>MALVPVGMAPRQMRVNRCIFASIVSFDACITYKSPCSPDAYHDDGWFICNNHLIKRFKMSKMVLPIFDEDDNQFKMTIARHLVGNKERGIKRILIPSATNYQDVFNLNSMMQAEQLIFHLIYNNENAVNTICDNLKYTEGFTSNTQRVIHSVYATTKSILDTTNPNTFCSRVSRDELRFFDVTNARALRGGAGDQLFNNYSGFLQNLIRRAVAPEYLQIDTEELRFRNCATCIIDETGLVASVPDGPELYNPIRSSDIMRSQPNRLQIRNVLKFEGDTRELDRTLSGYEEYPTYVPLFLGYQIINSENNFLRNDFIPRANPNATLGGGAVAGPAPGVAGEAGGGIAV[12x];>MNDSNSLLITRLAAQILSRNMQTVDVIVDDKTLSLEEKIDTLTSMVLAVNSPPQSPPRVTSSDLAASIIKNNSKMVGNDFEMRYNVLRMAVVFVKHYPKYYNETTAGLVAEIESNLLQYQNYVNQGNYQNIEGYDSLLNKAEECYVKIDRLFKESIKKIMDDTEAFEREQEAERLRAEQTAANALLERRAQTSADDVVNRADANIPTAFSDPLPGPSAPRYMYESSESDTYMETARRTAEHYTDQDKDYNAAYTADEYNSLVKTVLLRLIEKALATLKNRLHITTIDQLKKFRDYLNSDADAGEFQIFLNQEDCVILKNLSNLASKFFNVRCVADTLEVMLEALRNNIELVQPESDAVRRIVIKMTQEIKDSSTPLYNIAMYKSDYDAIKNKNIKTLFDLYNDRLPINFLDTSATSPVRKTSGKRSAEDDLLPTRSSKRANRPEINVISSEDEQEDDDVEDVDYEKESKRRKLEDEDFLKLKALEFSKDIVNEKLQKIIVVTDGMKRLYEYCNCKNSLETLPSAANYGSLLKRLNLYNLDHIEMNVNFYELLFPLTLYNDNDNSDKTLSHQLVNYIFLASNYFQNCAKNFNYMRETFNVFGPFKQIDFMVMFVIKFNFLCDMRNFAKLIDELVPNKQPNMRIHSVLVMRDKIVKLAFSNLQFQTFSKKDKSRNTKHLQRLIMLMNANYNVI[6x];>MKRIKCNKVRTVTEIVNSDEKIQKTYELAEFDLKNLSSLESYETLKIKLALSKYMAMLSTLEMTQPLLEIFRNKADTRQIAAVVFSTLAFIHNRFHPLVTNFTNKMEFVVTETNDTSIPGEPILFTENEGVLLCSVDRPSIVKMLSREFDTEALVNFENDNCNVRIAKTFGASKRKNTTRSDDYESNKQPNYDMDLSDFSITEVEATQYLTLLLTVEHAYLHYYIFKNYGVFEYCKSLTDHSLFTNKLRSTMSTKTSNLLLSKFKFTIEDFDKINSNSVTSGFNIYNFNK[6x];>MSAIALYLEINKLRLKIDEPMQLAIWPQLFPLLCDEHQSVQLNTDVLINFMMHVARKSQNTILNNNAAIASQYAAGNADVVAAPASAQPTPRPVINLFARANAAAPAQPSEELINMRRYRNAARKLIHHYSLNSTSSTEYKISDVVMTMIFLLRSEKYHSLFKLLETTFDDYTCRPQMTQVQTDTLLDAVRSLLEMPSTTIDLTTVDIMRSSFARCFNSPIMRYAKIVLLQNVALQRDKRTTLEELLIERGEKIQMLQPQQYINSGTEIPFCDDAEFLNRLLKHIDPYPLSRMYYNAANTMFYTTMENYAVSNCKFNIEDYNNIFKVMENIRKHSNKNSNDQDELNIYLGVQSSNAKRKKY[6x];>MECPFQIQVCISDRFFAFPHNLVEPQSDVGNKLIENLIVYVPTDDDRLYIDKKQFPKFNSVLVYRHEHDVNIDSRSPKKTASATIVYWNPLVPITEIGAGETRVFSVLLTNNLFYCNTMIVHHENPKCPIEFTYPETDMQSACSALLKNRNGQSVPPPIKSNLRPIACEIPLSHFKELVESNDFLLCFNLETSTMVKILSLKRIFCIFQYRKQPARYVINLPHEEIDNLYNKLNWERTRRLMKGDVPSNCATVNRSSLKYIKQAQSLLGIPDYSQTVVDFVKMFQKIIFPYQLVPNVIIKLNNFDQMVSSAPNKAEPYKKIRLFCKNDSIAISSSGIVPINMPDFSPPNTFDYSDYANRTNINFVTQRVLTDGGFSSGITVTPVKYNYYL[2x];>[2x]MSGGGNLLTLERDHFKYLFLTSYFDLKDNEHVPSEPMAFIRNYLNCTFDLLDDAVLMNYFNYLQSMQLKHLVGSTSTNIFKFVKPQFRFVCDRTTVDILEFDTRMYIKPGTPVYATNLFTSNPRKMMAFLYAEFGKVFKNKIFVNINNYGCVLAGSAGFLFDDAYVDWNGVRMCAAPRLDNNMHPFRLYLLGEDMAKHFVDNNILPPHPSNAKTRKINNSMFMLKNFYKGLPLFKSKYTVVNSTKIVTRKPNDIFNEIDKELNGNCPFIKFIQRDYIFDAQFPPDLLDLLNEYMTKSSIMKIITKFVIEENPAMSGEMSREIILDRYSVDNYRKLYIKMEITNQFPVMYDHESSYIFVSKDFLQLKGTMNAFYAPKQRILSILAVNRLFGATETIDFHPNLLVYRQSSPPVRLTGDVYVVDKNEKVFLVKHVFSNTVPAYLLIRGDYESSSDLKSLRDLNPWVQNTLLKLLIPDSVQ;>[2x]MASSLQSKWICLRLNDAIIKRHVLVLSEYADLKYLGFEKYKFFEYVIFQFCNDPQLCKIIENNYNYCMQIFKAPADDMRDIRHNIKRAFKTPVLGHMCVLSNKPPMYSFLKEWFLLPHYKVVSLKSESLTWGFPHVVVFDLDSTLITEEEQVEIRDPFVYDSLQELHEMGCVLVLWSYGSRDHVAHSMRDVDLEGYFDIIISEGSTVQEERSDLVQNSHNAIVDYNLKKRFIENKFVFDIHNHRSDNNIPKSPKIVIKYLSDKNVNFFKSITLVDDLPTNNYAYDFYVKVKRCPTPVQDWEHYHNEIIQNIMDYEQYFIK

To understand the provenance and biology of baculo-like viruses, we have determined the structure of the nucleocapsid in the intact BV of the prototypical baculovirus, Autographa californica multiple nucleopolyhedrovirus (AcMNPV). Using cryo–electron microscopy, we show that the nucleocapsid forms a covalently cross-linked helical tube protecting a highly compacted 134-kilobase pair DNA genome. The ends of the tube are sealed by the base and cap substructures, which share a 126-subunit hub but differ in components that promote actin tail–mediated propulsion and nuclear entry of the nucleocapsid, respectively. The nucleocapsid orchestrates key steps in the infection cycle including the packaging of the genome, membrane envelopment, actin tail–driven trafficking within the cells, and breach of the nuclear pore upon genome delivery.

The hub forms a ring with a 14-fold rotational symmetry (C14) consisting of five proteins that have various names in the literature for historical reasons. Here, we rename them Hub1 (ODV/BV-C42 or AC101), Hub2 (ODV-EC27 or AC144), Hub3 (VP80 or AC104), HSP1 (hub spike protein 1, AC109), and HSP2 (hub spike protein 2, AC142) according to their functions. Hub1 and Hub2 form an intricate complex, with the compact Hub2 at its core and a series of helices in the C terminus of Hub1 (D3239-350) wrapping around most of Hub2. In the base, but not the cap, the hub accommodates a large chamber-like structure that forms a “plug” (bottom middle). Like the core of the hub, the plug is composed of Hub1-Hub2 complexes. Relative to the Hub2 orientation in the hub, the inner Hub2 subunit rotates by 162° toward the central axis of the particle due to a sharp kink in the handle of the other Hub2 subunit. This conformational shift effectively closes the chamber-like structure, sealing the basal end of the nucleocapsid. The inner side of the hub is decorated by 14 copies of the baculovirus C-terminal domain (CTD) phosphatase (BCP; also known as 38K or AC98) protein, which was not known to be a structural component of the nucleocapsid before an independent structure of the ODV. Sequence and structural analyses identify BCP as a member of the haloacid dehydrogenase (HAD)-like superfamily of phosphatases. BCP is positioned on the inner side of the base, with a fully accessible active site facing the genomic DNA.>[4x]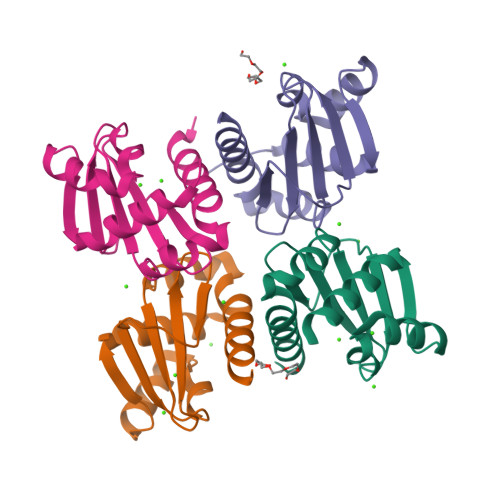MELHHHHHHEEMPFKPLVTAGIESLLNTFLYRSPALKTARSRLLGKVLRVEVKGFSTSLILVFSERQVDVLGEWAGDADCTVIAYASVLPKLRDRQQLTALIRSGELEVQGDIQVVQNFVALADLAEFDPA Phytochromes sense ambient light levels in plants, fungi, and bacteria. The proteins detect light and trigger intracellular signalling cascades, which regulate many light-dependent phenotypes. The PAS and GAF domains hold a tetrapyrrole bilin chromophore, represented by phytochromobilin, phycocyanobilin, or biliverdin in plants, cyanobacteria, or bacteria, respectively. Upon light absorption by the chromophore, a sequence of structural changes is initiated, which shuttles the protein from a red light-absorbing state (Pr) to a far-red light-absorbing state (Pfr) or vice versa.

The PAS-GAF fragment of the D. radiodurans phytochrome was crystallised in essentially the same conditions but the cryoprotectant 2-methyl-2, 4-pentanediol was added directly to the crystallisation buffer. Those changes resulted in the protein packing as monomers instead of dimers in contrast to previously published conditions. The space group C121 and cell dimensions were highly similar to the crystals from monomeric PAS-GAF21. We recorded diffraction data at cryogenic conditions at the European Synchrotron Radiation Facility (ESRF) and solved the structure to 1.35 Å resolution by molecular replacement with 4Q0H9 as a search model. We refer to this structure as “LowT”. The 1.35 Å resolution to which the LowT structure has been determined is the highest reported so far for a wild-type PAS-GAF fragment. We also note that the LowT data support a water molecule with partial occupancy close to Tyr263. The water is hydrogen-bonded to the A-ring carbonyl, the pyrrole water and the functionally important Asp207. The diffuse electron density in the LowT structure could be due to radiation damage or to alternate conformations of the chromophore-protein bond. Importantly, the LowT structure corroborates the SFX structures.

> MASMTGGQQMGRGSMSRDPLPFFPPLYLGGPEITTENCEREPIHIPGSIQPHGALLTADGHSGEVLQMSLNAATFLGQEPTVLRGQTLAALLPEQWPALQAALPPGCPDALQYRATLDWPAAGHLSLTVHRVGELLILEFEPTEAWDSTGPHALRNAMFALESAPNLRALAEVATQTVRELTGFDRVMLYKFAPDATGEVIAEARREGLHAFLGHRFPASDIPAQARALYTRHLLRLTADTRAAAVPLDPVLNPQTNAPTPLGGAVLRATSPMHMQYLRNMGVGSSLSVSVVVGGQLWGLIACHHQTPYVLPPDLRTTLEYLGRLLSLQVQVKEALEHHHHHH>[2x]A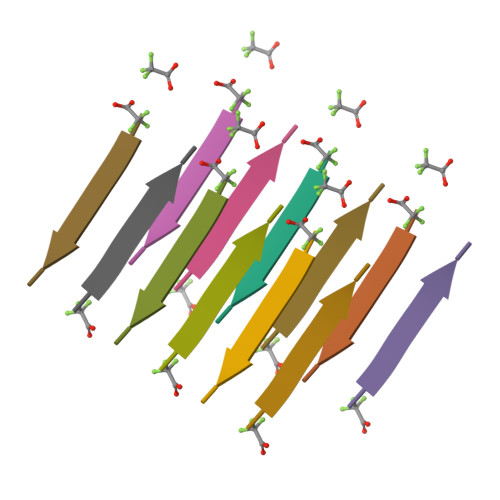ALALL> MADCTFTQLEIVPQFGSPNMFGGEDEHVRVMFS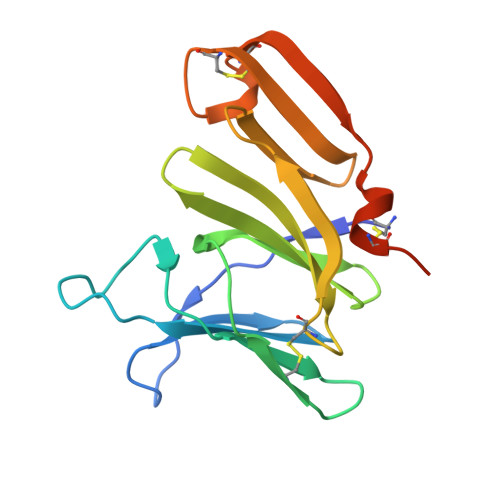NEDPNDDNPDAFPEPPVYLADRDSGNDCRIEDGGIWSRGGVFLSQDGRRVLMHEFSGSSAELVSYDSATCKVVHREDISGQRWAVDKDGLRLGQKCSGESVDSCAKIVKRSLAPFCQTAKKLEHHHHHH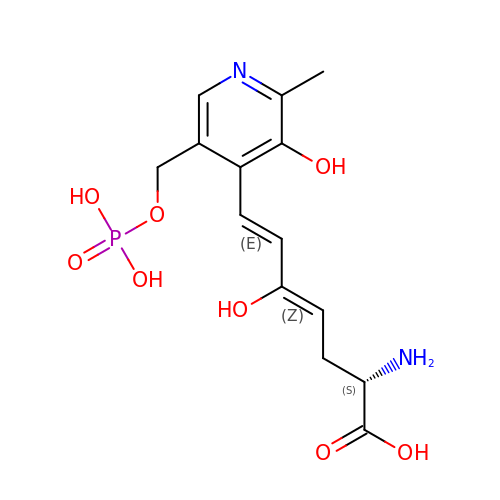1-AMINO-7-(2-METHYL-3-OXIDO-5-((PHOSPHONOXY)METHYL)-4-PYRIDOXAL-5-OXO-6-HEPTENATE | C14 H19 N2 O8 P | FKVMVCAAQIJMAO-UGEYCXAUSA-N> KETAAA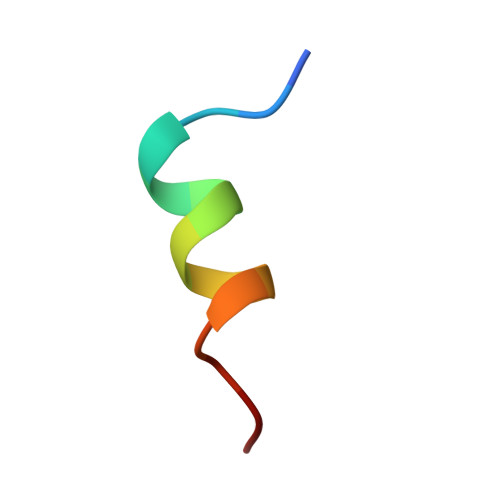KFERQHMDS>[8x]SMRNVALITGITGQDGSYLAEFLLEKGYEVHGIVRRSSSFNTGRIEHL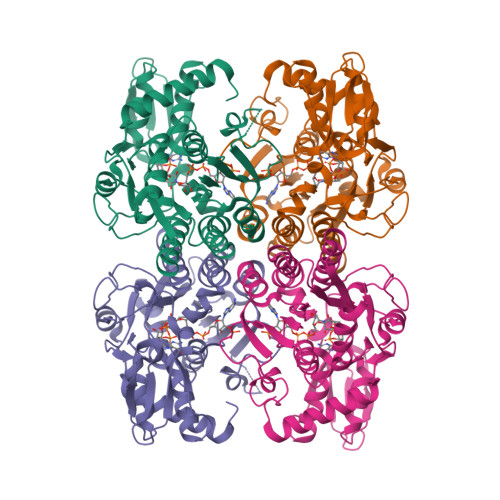YKNPQAHIEGNMKLHYGDLTDSTCLVKIINEVKPTEIYNLGAQSHVKISFDLAEYTADVDGVGTLRLLDAVKTCGLINSVKFYQASTDELYGKVQEIPQKETTPFYPRSPYGAAKLYAYWIVVNFREAYNLFAVNGILFNHESPRRGANFVTRKISRSVAKIYLGQLECFSLGNLDAKRDWGHAKDYVEAMWLMLQNDEPEDFVIATGEVHSVREFVEKSFLHIGKTIVWEGKNENEVGRCKETGKVHVTVDLKYYRPTEVDFLQGDCTKAKQKLNWKPRVAFDELVREMVHADVELMRTNPNA> GPLGSRKSSHLILSSIVSLALVGVTPLSVLADSKQDINQYFQSLTYEPQEILTNEGEYIDNPPATTGMLENGRFVVLRREKKNITNNSADIAVIDAKAANIYPGALLRADQNLLDNNPTLISIARGDLTLSLNLPGLANGDSHTVVNSPTRSTVRTGVNNLLSKWNNTYAGEYGNTQAELQYDETMAYSMSQLKTKFGTSFEKIAVPLDINFDAVNSGEKQVQIVNFKQIYYTVSVDEPESPSKLFAEGTTVEDLKRNGITDEVPPVYVSSVSYGRSMFIKLETSSRSTQVQAAFKAAIKGVD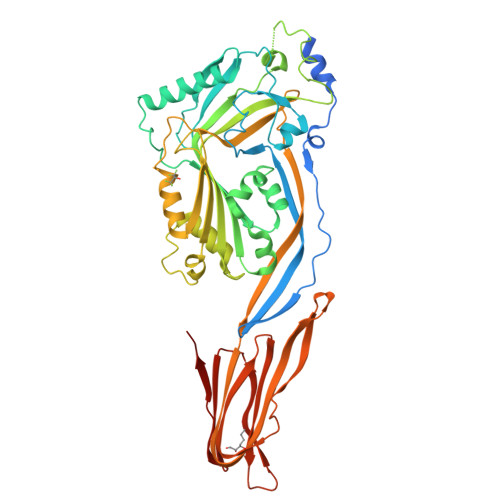ISGNAEYQDILKNTSFSAYIFGGDAGSAATVVSGNIETLKKIIEEGARYGKLNLGVPISYSTNFVKDNRPAQILSNSEYIETTSTVHNSSALTLDHSGAYVAKYNITWEEVSYNEAGEEVWEPKAWDKNGVNLTSHWSETIQIPGNARNLHVNIQECTGLAWEWWRTVYDKDLPLVGQRKITIWGTTLYPQYADEVIELERPHRD>[5x]QEEGEDNGGEDNKKLRGALSSAILSEKPNVKWEDVAGLEGAKEALKEAVILPVKFPHLFKGNRKPTSGILLYGPPGTGKSYLAKAVATEANSTFFSVSSSDLVSKWMGESEKLVKQLFAMARENKPSIIFIDEVDALTGTRGEGESEASRRIKTELLVQMNG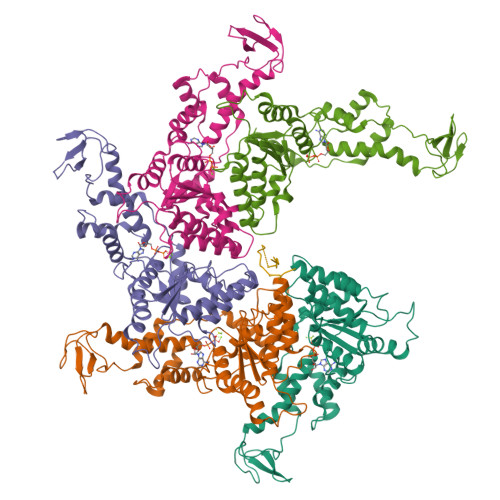VGNDSQGVLVLGATNIPWQLDSAIRRRFERRIYIPLPDLAARTTMFEINVGDTPCVLTKEDYRTLGAMTEGYSGSDIAVVVKDALMQPIRKIQSATHFKDVSTEDDETRKLTPCSPGDDGAIEMSWTDIEADELKEPDLTIKDFLKAIKSTRPTVNEDDLLKQEQFTRDFGQEGN> MGQLTQTNKTELGVFDDMNQAIEAAKEAQLVVKKMSMDQREKIISAIRKKTIEHAETLARMAVEETGMGNVGHKILKHQLVAEKTPGTEDITTTAWSGDRGLTLVEMGPFGVIGAITPCTNPSETIICNTIGMLAGGNTVVFNPHPAAIKTSNFAVQLINEASLSAGGPVNIACSVRKPTLDSSKIMMSHQDIPLIAATGGPGVVTAVLQSGKRGIGAGAGNPPVLVDETADIRKAAEDIINGCTFDNNLPAIAEKEVVAIDAIANELMNYMVKEQGCYAITKEQQEKLTNLVITPKGLNRNCVGKDARTLLGMIGIDVPSNIRCIIFEGEKEHPLISEELMMPILGIVRAKSFDDAVEKAVWLEHGNRHSAHIHSKNVDRITTYAKAIDTAILVKNAPSYAAIGFGGEGFCTFTIASRT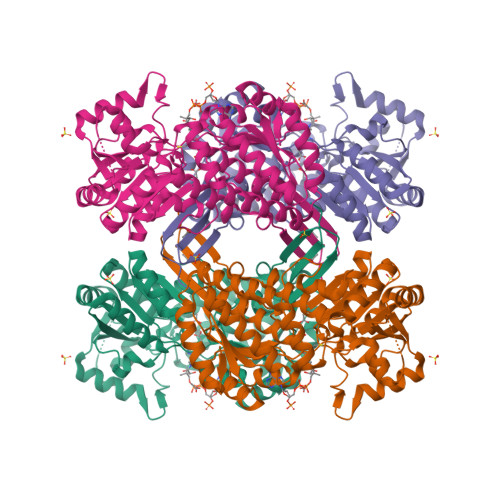GEGLTSASTFTKRRRCVMSDSLCIR> SMSVPQTKAELLLAIDKNFSKLISYLNTIPPEITSDKSMDGHAKGTEMSVRDLVSYLLGWNALVVKWIASDAKGLPVDFPETGYKWNQLGLLAQKFYSDYSELSYELLVAELQTVKNEIVNLINDRTDDILYGRPWYTKWTMGRMISFNTSSPYANANGRLRKWAKNNNISLK

The precursor PdDfsB is cleaved by subtilisin to yield biologically active Slf, and the chemical gradients of both proteins between two growing colonies could be accurately modelled. However, remarkably, the dfsB gene is widely distributed across Gram-positive and to some extent Gram-negative bacterial kingdoms (PFAM entry DUF1706). PdDfsB adopts a four-helical bundle core structure that belongs to the DinB structural superfamily. The most strongly conserved region of PdDfsB is the C-terminal helix, which is present within the mature Slf sequence.

The second, related clade contains DfsB homologues from mainly Gram-negative bacteria, again including many pathogens. We were able to express, purify and obtain crystal structures for DfsB homologues from Clostridium difficile 630 and Escherichia coli UTI89, as well as of IRC4 from S. cerevisiae. For the purposes of clarity, we refer to the first two proteins as CdDfsB and EcDfsB, respectively; however, we have no evidence that they are truly acting as DfsB homologues by undergoing cleavage and release of their analogous Slf “toxin”. The overall structures of CdDfsB, EcDfsB and IRC4 are identical with that of PdDfsB, with strong conservation of overall topology and surface charge, particularly in the C-terminal helix.> EEKAIDARNLFEYHCAKCHGLTGEANKRGKALK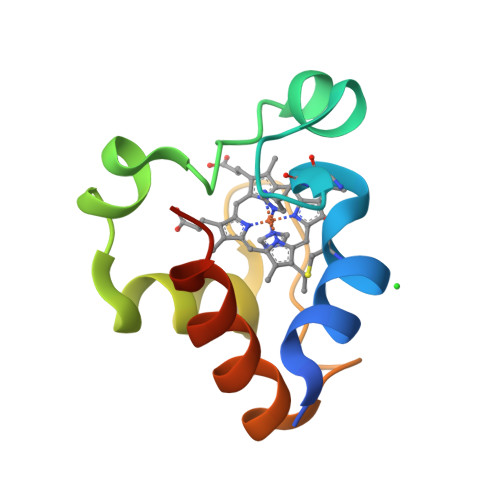APDLCDPGWQNSKTDKEILYSITNGKNKMPAWNERLTPEEIEALARYVRKLSKKQR2-aminoethyl 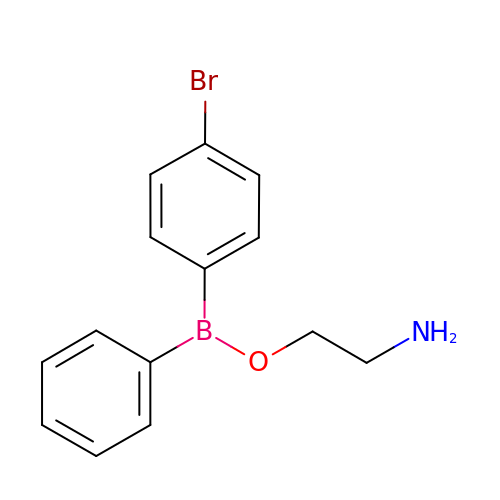(4-bromophenyl)phenylborinate | C14 H15 B Br N O | WVCHSOYKLDCILQ-UHFFFAOYSA-N> MDGTAAEPRPGAGSLQHAQPPPQPRKKRPEDFKFGKILGEGSFSTTVLARELATSREYAIKILEKRHIIKENKVPYVTRERDVMSRLDHPFFVKL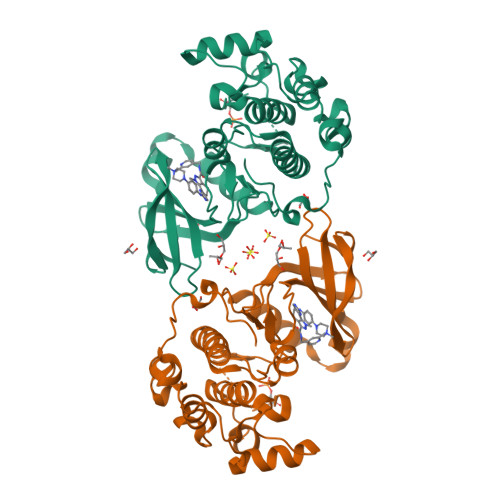YFTFQDDEKLYFGLSYAKNGELLKYIRKIGSFDETCTRFYTAEIVSALEYLHGKGIIHRDLKPENILLNEDMHIQITDFGTAKVLSPESKQARANSFVGTAQYVSPELLTEKSACKSSDLWALGCIIYQLVAGLPPFRAGNEYLIFQKIIKLEYDFPEKFFPKARDLVEKLLVLDATKRLGCEEMEGYGPLKAHPFFESVTWENLHQQTPPKLT> MSLSNKLTLDKLDVKGKRVVMRVDFNVPMKNNQITNNQMIKAAVPSIKFCLDNGAKSVVLMSHLGRPDGVPMPDKYSLEPVAVELKSLLGKDVLFLKDCVGPEVEKACANPAAGSVILLENLRFHVEEEGKGKDASGNKVKAEPAKIEAFRASLSKLGDVYVNDAFGTAHRAHSSMVGVNLPQKAGGFLMKKELNYFAKALESPERPFLAILGGAKVADKIQLINNMLDKVNEMIIGGGMAFTFLKVLNNMEIGTSLFDEEGAKIVKDLMSKAEKNGVKITLPVDFVTADKFDENAKTGQATVASGIPAGWMGLDCGPESSKKYAEAVTRAKQIVWNGPVGVFEWEAFARGT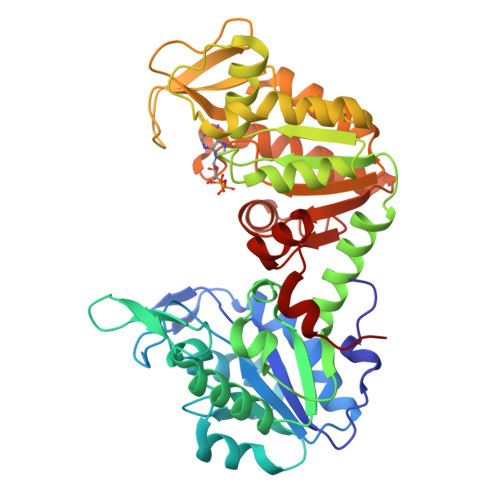KALMDEVVKATSRGCITIIGGGDTATCCAKWNTEDKVSHVSTGGGASLELLEGKVLPGVDALSNI>MKIGIIGAMQQEVAILKDLIEDVQEVNQAGCTFYSGQIQGVDVVLLQSGIGKVSAALGTALLISQYAPDVVINTGSAGGFDASLNVGDVVISSEVRHHDADVTAFGYEIGQMAGQPAAFKADEKLMTVAEQALAQLPNTHAVRGLICTGDAFVCTAERQQFIRQHFPSVVAVEMEASAIAQTCHQFKVPFVVVRAISDVADKESPLSFEEFLPLAAKSSSAMVLKMVELLK[2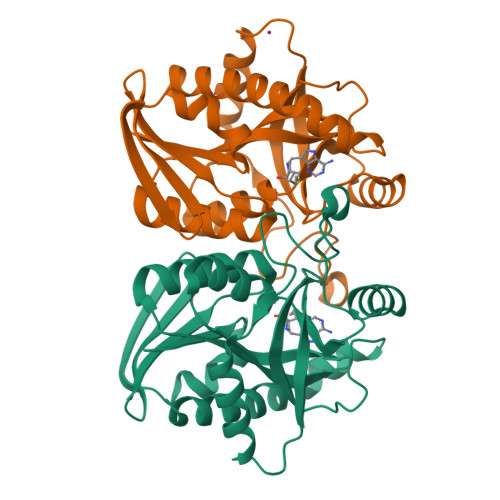x]>[3x]HHHHHHSSGLVPRGSHMMNPFHDLEPGPNVPEVVYALIEIPKGSRNKYELDKETGLLKLDRVLYT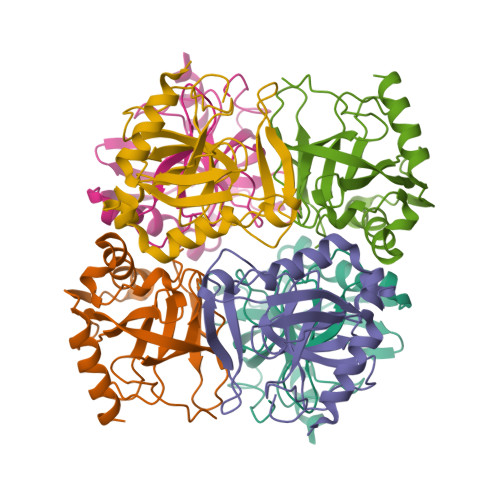PFHYPVDYGIIPRTWYEDGDPFDIMVIMREPTYPLTIIEARPIGLFKMIDSGDKDYKVLAVPVEDPYFKDWKDISDVPKAFLDEIAHFFKRYKELEGKEIIVEGWEGAEAAKREILRAIEMYKEKFGKKE> MLNRSRLRRVWLGGTAANTSLGRDVMPSTGKYINIVSPTDVAANISAGAMPPEANVA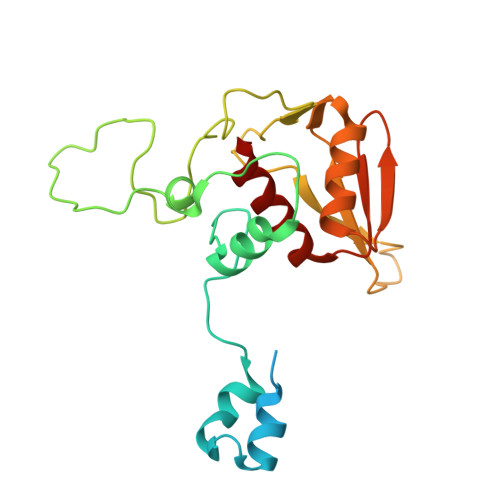AALPVPRIQYSKWNRALRSDVYDELLKLPLRYKLHDFAKLCPPQRCQEEPEAVGVVGRDSAVGYLPPLGPADPLDTIPFFVHRSSNGVLPGKVFSMHPRNLMPAFYLRIQQVEGDMFRFEEELLKIFPTKKIFVRSHSIYVYNVALDGRMVLHHWLLGLGF> MSNFAI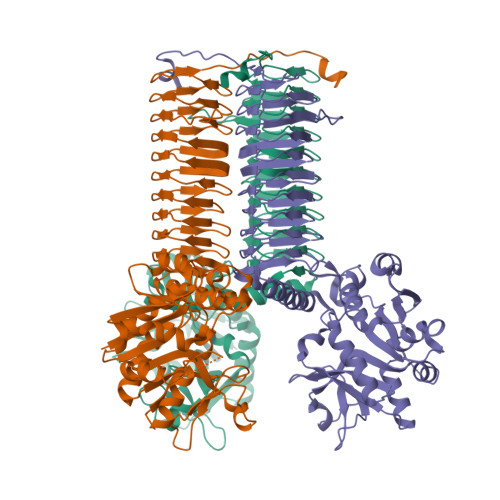ILAAGKGTRMKSDLPKVLHKVAGISMLEHVFRSVGAIQPEKTVTVVGHKAELVEEVLAGQTEFVTQSEQLGTGHAVMMTEPILEGLSGHTLVIAGDTPLITGESLKNLIDFHINHKNVATILTAETDNPFGYGRIVRNDNAEVLRIVEQKDATDFEKQIKEINTGTYVFDNERLFEALKNINTNNAQGEYYITDVIGIFRETGEKVGAYTLKDFDESLGVNDRVALATAESVMRRRINHKHMVNGVSFVNPEATYIDIDVEIASEVQIEANVTLKGQTKIGAETVLTNGTYVVDSTIGAGAVITNSMIEESSVADGVIVGPYAHIRPNSSLGAQVHIGNFVEVKGSSIGENTKAGHLTYIGNCEVGSNVNFGAGTITVNYDGKNKYKTVIGNNVFVGSNSTIIAPVELGDNSLVGAGSTITKDVPADAIAIGRGRQINKDEYATRLPHHPKNQ2-(3-benzyl-5-bromo-1H-indol-1-yl)-N-hydroxyacetamide | C17 H15 Br N2 O2 | 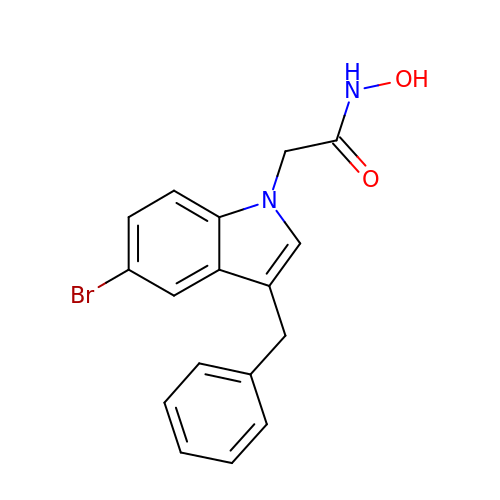UALZWYXMMCSOBJ-UHFFFAOYSA-N>SGSHMTMGTVNHQPLLTQADLLKRGLADLQEHDAELARILDAEVARQQRTLSLVASCCAVKPRTLAASSSALVNVTAEGVPGRRYHAGCENVDLVESLAIQRARELFGAQYAGVQSHSASSANYQVLAALLEPGDTLLGMALDNGGHLTHGSPVTFSGTYYKAIGYGTTKEGLIDYDEVRRLALEHRPRLIICGATAYSRVVDFERFRQIADEAGAILMADISHIAGLVATGRHPSPIDAAHVTTTCTHKQLVGPRGGLILSGRDANEKVPGRDATFSRVLELAVFPRMQGAPAVNMMAAKAAALGYAMTPEFDAEMQRIRDAADVMASEFQARDYEVVGGRSENHTILIRLRAAMTGAIAETALEHCGIVVNKNRVPGETRSSFVTSGLRIGTGALAQRHVDAQGCRQIVDLLCRILDEVTPLGESEFTLDPALRKQFCAEAEALCVKYPIADYLAILE[2x]

While GlyA from E. coli, one of the best‐studied examples, catalyzes reversible conversion between serine and glycine and thereby affords mTHF as the major source of C1 unit in cells, the newly identified PbzB involved in the benzobactin biosynthesis catalyzes production of 2‐hydroxymethylserine using l‐serine, d‐serine, or glycine. PbzB has high sequence similarity with AsmD and FmoH, and contains a conserved PLP‐binding loop in which the lysine residue forms a Schiff base with PLP. PbzB, same as GlyA‐type enzymes, forms homodimers with two active sites shared between the two monomers.

To gain an insight into the substituted residues involved in substrate binding in PbzB, we set out to structurally analyze its apo‐ and substrate‐bound form. While crystals of the apo‐form diffracted to 2.8 Å, we only obtained poorly diffracting anisotropic crystals for PbzB co‐crystallized with l‐serine and mTHF. However, the residues coordinating PLG and mTHF were not visible in the PbzB structure, since they were probably too flexible in the absence of a ligand, and therefore, we modeled PbzB using Alphafold. The simulated structural model had a confidence of over 95 % and an RMSD of 0.97 and 0.84 for the crystal structures of apo‐PbzB and GlyA from E. coli, respectively. An in‐depth analysis of the active sites revealed that all residues involved in substrate binding within GlyA and PbzB are superimposable. Even Y55 and Y65 in GlyA are superimposable with T68 and H78 in PbzB, but these alterations might enlarge the binding pocket of PbzB. While Y55 and Y65 in GlyA perfectly coordinate PLG, T68 and H78 in PbzB open the space for the binding of PLS. Particularly, the substitution of Y55 by T68 may lead to a reduction of negative charges in the binding pocket and thus enable coordination of serine bound to PLP. However, the PbzB T68Y H78Y mutant did not catalyze formation of any detectable amount of serine or 2‐hydroxymethylserine, suggesting that T68 and H78 residues are crucial to maintaining the function of PbzB. Therefore, one could assume that benzobactin‐producing bacteria remodel an enzyme from the central amino acid metabolism to deliver a building block for the NRPS biosynthetic pathway.> QHLMCEEHEEEKINIYCLSCEVPTCSLCKVFGAHKDCEVA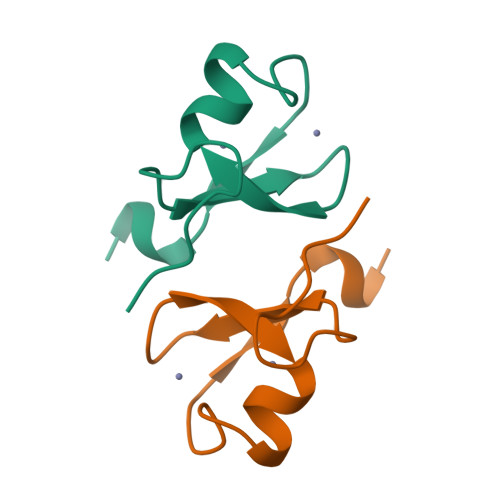PLPTIYK>[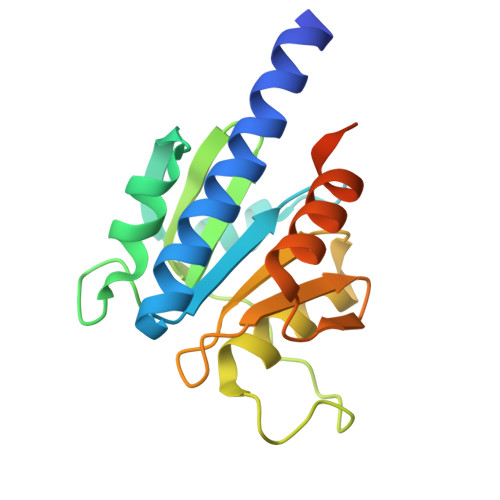2x]GPLGSYGSRIEREQHHLIESIEKSTQYMAKRRIGALISVARDTGMDDYIETGIPLNAKISSQLLINIFIPNTPLHDGAVIIKGNEIASAASYLPLSDSPFLSKELGTRHRAALGISEVTDSITIVVSEETGGISLTKGGELFRDVSEEELHKILLKELVTVTAKKPSIFSKWKGGKSE>MGRILVIEDEISLNKTIIDNLNEFGYQTDSSENFKDGEYFIGIRHYDLVLASWNLPDGDGAELVNTIKHKSPRTSVMIMSAKADKDTEIKALKAGADDFVKKPLDFDILLARIEARLRLGGTNVIKIEDLVIDPDEEKITYKGQDIELKGKPFEVLTHLARHSDQIVSKEQLLDAIWEEPELVTPNVIEVAINQIRQKMDKPLNISTIETVRRRGYRFCFPKKS[2x]

The C. jejuni CosR regulator is essential to the viability of this bacterium and is responsible for regulating the expression of a number of oxidative stress defense enzymes. Importantly, it also modulates the expression of the CmeABC multidrug efflux system, the most predominant and clinically important system in C. jejuni that mediates resistance to multiple antimicrobials. CosR belongs to an OmpR/PhoB family of response regulators. We determined that CosR assembles as a homodimer with each CosR protomer contributing to major conformational changes to facilitate DNA binding.

Interestingly, we indeed observed single-particle images of free CosR (apo-CosR), CosR-DNA, and free DNA. The apo-CosR regulator assembles as a symmetric dimer with both subunits displaying identical conformational states. We finally refined cryo-EM structures of this apo-CosR dimer to a resolution of 3.77 Å. The final model of each subunit contains residues 1–120, 126–143, and 151–161. The cryo-EM structure of apo-CosR indicates that CosR can be divided into two domains, an N-terminal receiver domain (RD) and a C-terminal DNA-binding domain (DBD), similar to those found in the X-ray structures of the Thermotoga maritima DrrB, T. maritima DrrD, and Mycobacterium tuberculosis MtrA regulators. Residues 1–116 create the RD, whereas residues 124–221 form the DBD. All of the N-terminal RD residues are clearly visible in the apo-CosR structure; however, many of the C-terminal DBD residues, such as residues 162–221, are imperceptible with no observable cryo-EM densities. Residues 117–123 likely form a flexible linker region to directly connect the RD and DBD. Based on the structural information, apo-CosR is very flexible in nature, particularly the C-terminal DBD. However, our cryo-EM structure of apo-CosR indicates that CosR is in a dimeric form in solution.> MKQKINKLLKNKGVQDKYKYLSKLILLDQEIKGKIKRKNKKEKQKRKNKLILEEMQNTTNIVHVPVHMGHTHYFDYIDSFPKLKEGPTLEENHITNQKILREQLISGQQ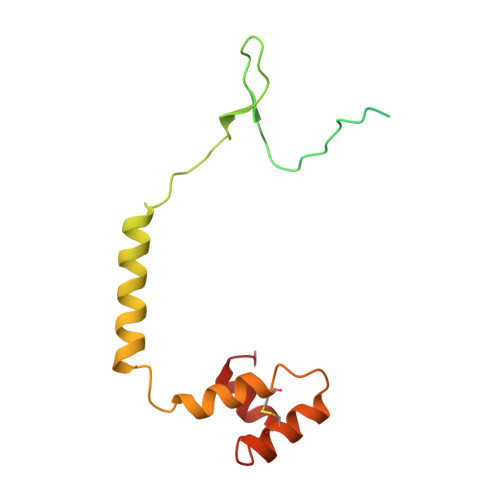GLEQNLCLRNCFKLSQKRYIEFCLDRKCGGADFQRAATILGYTKN> MTKKSASSNNKVVATNRKARHNYT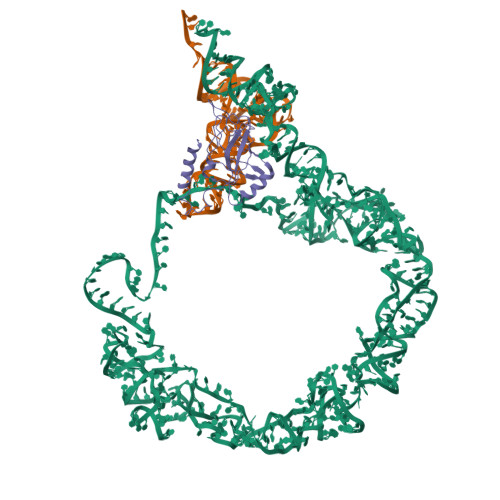ILDTYEAGIVLMGTEVKSLREGQASLADAFATVDDGEIWLRNVHIAEYHHGTWTNHAPRRNRKLLLHRKQIDNLIGKIRDGNLTLVPLSIYFTDGKVKVELALARGKQAHDKRQDLARRDAQREVIRELGRRAKGKI>HHHHHHASVMNINQEQLLMFQAVMETGSFSAAARKLGKVPSAVSMSIANLEIDLNLTLFERKGR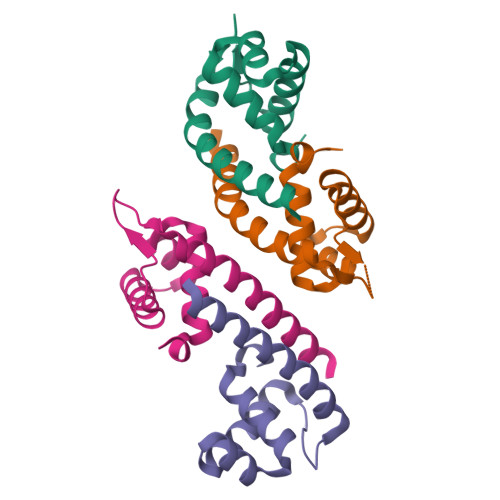EPTPTAEARVLYEKTAQLLIEMNQWKQHAHAL[4x]>[4x]GPHMAAAAMAAAAGGGAGAARSLSRFRGCLAGALLGDCVGSFYEAHDTVDLTSVLRHVQSLEPDPGTPGSERTEALYYTADTAMARALVQSLLAKE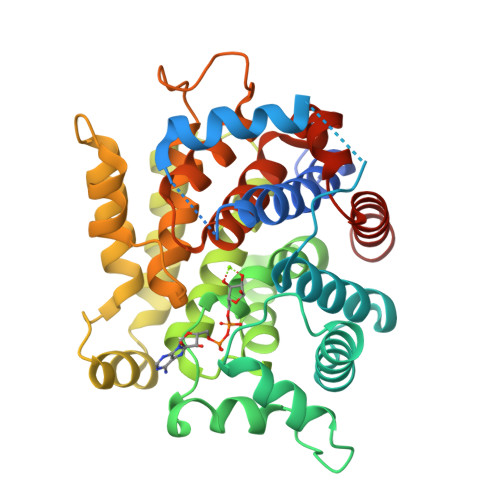AFDEVDMAHRFAQEYKKDPDRGYGAGVVTVFKKLLNPKCRDVFEPARAQFNGKGSYGNGGAMRVAGISLAYSSVQDVQKFARLSAQLTHASSLGYNGAILQALAVHLALQGESSSEHFLKQLLGHMEDLEGDAQSVLDARELGMEERPYSSRLKKIGELLDQASVTREEVVSELGNGIAAFESVPTAIYCFLRCMEPDPEIPSAFNSLQRTLIYSISLGGDTDTIATMAGAIAGAYYGMDQVPESWQQSCEGYEETDILAQSLHRVFQKS>[2x]MSTAAEGGAIRRAGHEPRYDLAQLPPAPPTTVAVIEGMATGAPQRVVAQADAAARVSELFVDPQQRERISRIYDKTRIDTRRMAVDPLDDEFDEFRREPATIRDRMNLFYQHAVPLAVDVAARALDGLPYAPDEIGQLVFVTSTGFIAPGVDVEIVKQLGLPRSISRVVVNFMGCAAAMNAIRTATNYVRAHPSMKALVVCIELSSVN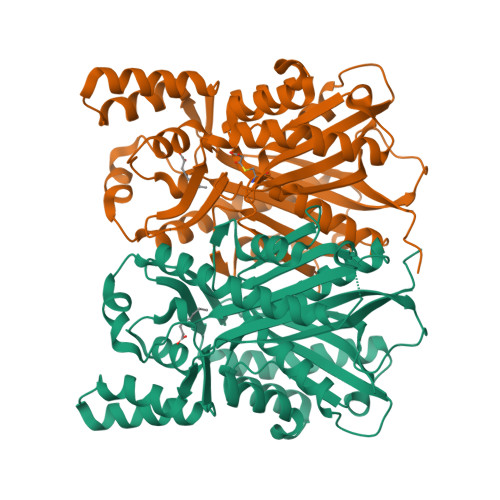AVFADDINDVVIHSLFGDGCGALVIGASQVQQPLPAGNVVIRSSFSQLLDDSEDGIVLGVNHDGITCELSENLPSYIYRSVDPVVAEMLRDNGLSKADIDLWAIHPGGPKIIEQSARSLGIPVGRAVQSWDVLAQFGNMLSVSLIFVLEMMVAQAESDKPISTGVAFAFAPGVTVEGMLFDIIRRGNSSSVDKLAAALEHHHHHH N-Methyl-6-(1,3-dihydroxy-isobutyl)thymine 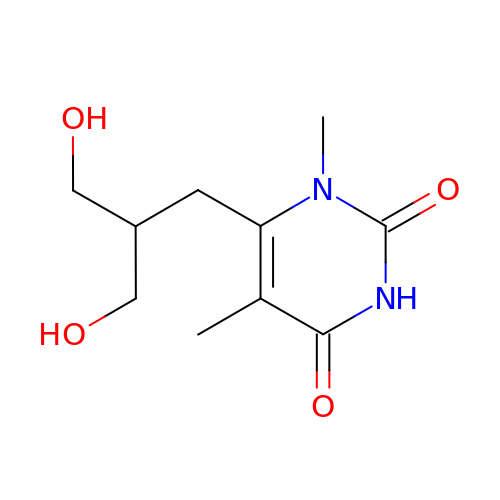| C10 H16 N2 O4 | FMPCUJIPAJPVKR-UHFFFAOYSA-N>[4x]GHMFQCNVPLGMESGRIANEQISASSTYSDGRWTPQQSRLHGDDNGWTPNLDSNKEYLQVDLRFLTMLTAIATQGAISRETQNGYYV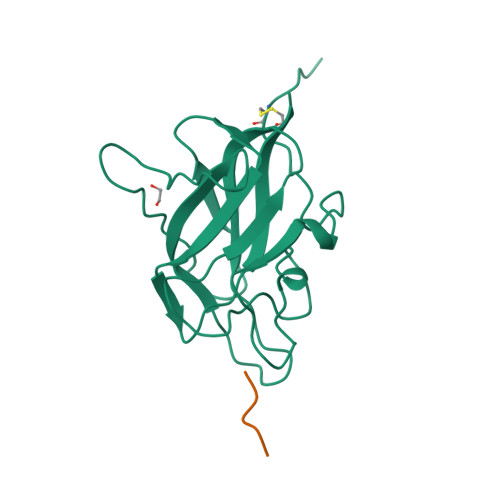KSYKLEVSTNGEDWMVYRHGKNHKVFQANNDATEVVLNKLHAPLLTRFVRIRPQTWHSGIALRLELFGCRVTSGS;>[3x]RKLRR> VPFFMI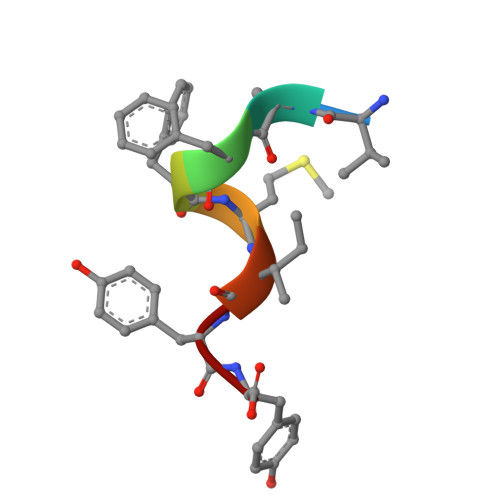YY> MSSVSVHYSTHKINKVRFLNRNFHNDTSLFVTGTNHPVLSKNKISVWGLESRQNSDEIEELASVPIDGIVTELKVIEINNKPMIIGSTSKGSIFMYSIFNLPNKFEYIGYDGLLDKKYENYNNINNINDTYDTCNLLKERIWFNSSSNNNNVNSNNINNNNYNNNNNNYNNNNNNNNNNNNNNNNNNNNGSCINSFDISYDQHSLVTVGNDGVMNLLSIENLIPIYTNRYIDGLSVNVVKSITSNQIITSGELGRYIKFWDIRSNSSQPV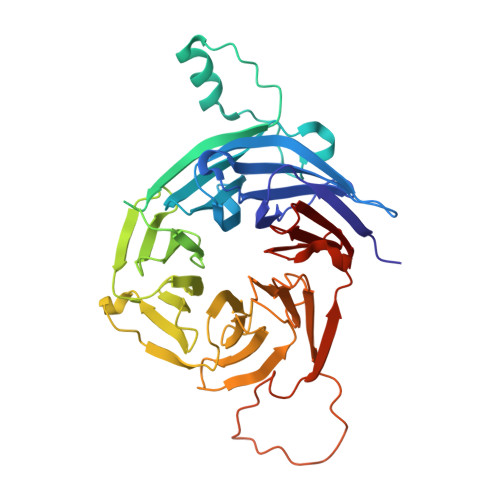KTIKTQCPRIFSLAIHKDEQHIIAAGSSDGQVNLFDIRNDYSIDQNKTHNSNVWELSFSKSNPNQLYSCSEDGFIYQYSYNKDNLGGGGMMTLPNQINNTFDIYSKEVSLLQLPTSIGSIDSFDINSNINRLICCSTSSQCLIVKSL>[2x]GSHMNTAEEDMEDDTSWRSEATFQFTVERFSRLSESVLSPPCFVRNLPWKIMVMPRFYPDRPHQKSV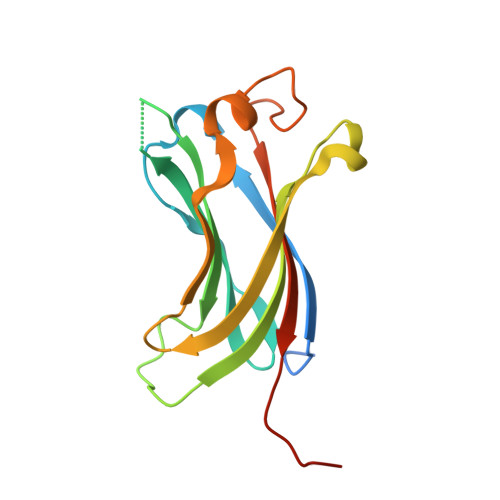GFFLQCNAESDSTSWSCHAQAVLKIINYRDDEKSFSRRISHLFFHKENDWGFSNFMAWSEVTDPEKGFIDDDKVTFEVFVQADAPGGSRAHSSH>[8x]MVKNWLFGKKRKEDADALATLKGQQNRLQAEARNLERQSDEQKILASKMLKAGNKAGARQALKRRAVFMKR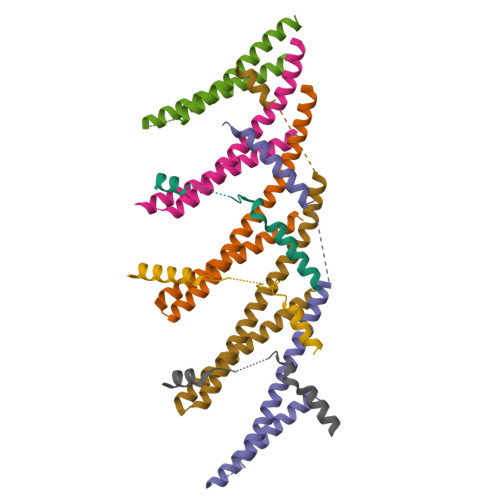LNTVHNTAMNLQAQIDSIQTATSTAETVKAMELGTKVVGEKIKTVSPERTERVMDSVMEQRDQIEMMTEALSDPSLSEGILDFEDDAAIDEQLAQLEAEMDLGTTTSLPDVSGLPSTPVGTGEKEEDTSELEAELEGLKKKMSEDKQ> VRATGHSYEKYNNWETIEAWTQQVATENPALISRSVIGTTFEGRAIYLLKVGKAGQNKPAIFMDCGFHAREWISPAFCQWFVREAVRTYGREIQVTELLNKLDFYVLPVLNIDGYIYTWTKSRFWRKTRSTHTG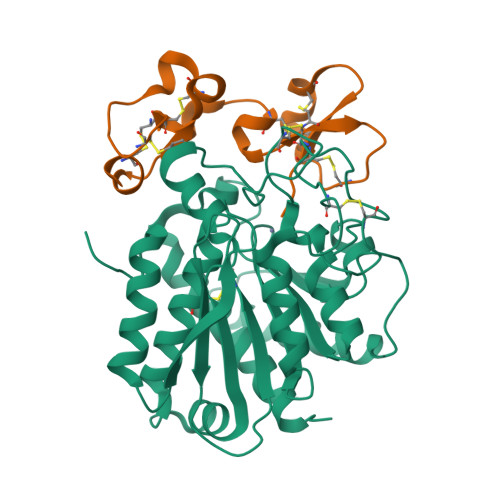SSCIGTDPNRNFDAGWCEIGASRNPCDETYCGPAAESEKETKALADFIRNKLSSIKAYLTIHSYSQMMIYPYSYAYKLGENNAELNALAKATVKELASLHGTKYTYGPGATTIYPAAGGSDDWAYDQGIRYSFTFELRDTGRYGFLLPESQIRATCEETFLAIKYVASYVLEHLY;> NECVSKGFGCLPQSDCPQEARLSYGGCSTVCCDLSKLTGCKGKGGECNPLDRQCKELQAESASCGKGQKCCVWLH>GHENEISIKIETYLQEEYGEEFEVLSWNQPKLLPSDNGAIYATCISKNDPKHPFEGSYFNPEEPNSEIEIIYDGYGQRLLAKQMESMIEEAISQAAENYYIQGDIIIPEEWQDIPVEEISQWKNYVDLCNQSNSDYKTLGSAWVYIDASTMKGKTDEEEYQMYEEVYRDKLGGQALLYVYYLDHKSFEKAEKILEIFTSGDEGSNFEDIIEGQPYFGTIMRYGSD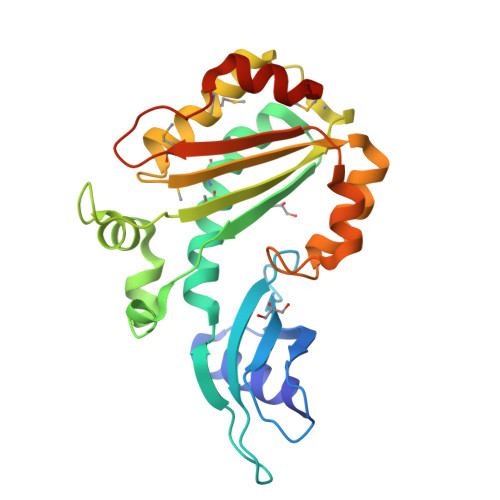KFDDNLEIFKAAKQGKEQEKYQ[2x]> GSHMRKQL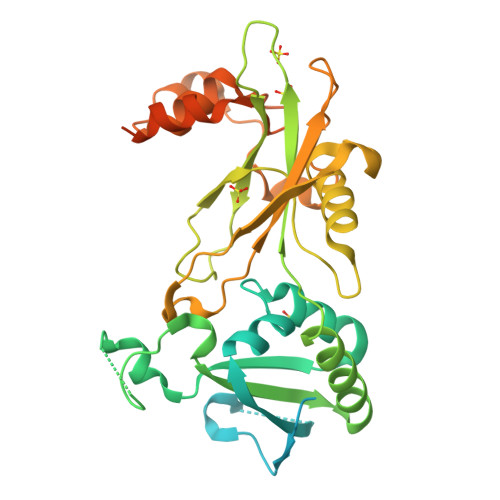FFTLARPCVAVGRRFISGDNKSIDSSAFISDDDALRGELASALDTEGHALPFDVHLQQPHSSGDGTAGDTSTIQLEKLSHPPARFDLLTNSFVYKWQTKAALARKVSGPMREWAAELKYRTGVHIELEPTYPERLSENAVKGSGSDDGDGTQWGAYETADDVDITVYLFGSERGIFNCHKLMEAAIQQDPVYVRLGIFRRLANSSEVEWLMLRRINRELRPPDIPPISLKLPGKWTLLYERYKEAAIRTLWEETGITVDASNVYPTGHLYQTVPQYYWRVPVRYFVAEVPSDIRVEGPQVVPLQYMRNWDARLLRQSPDPIDRAWAQLADPATGCAWMKASMIDQLQKPLRGDNYMAIRYTPPPYSNLQEVVGLGDGSITPSTGNGEDAS>[3x]MPKIYTKTGDKGFSSTFTGERRPKDDQVFEAVGTTDELSSAIGFALELVTEKGHTFAEELQKIQCTLQDVGSALATPCSSAREAHLKYTTFKAGPI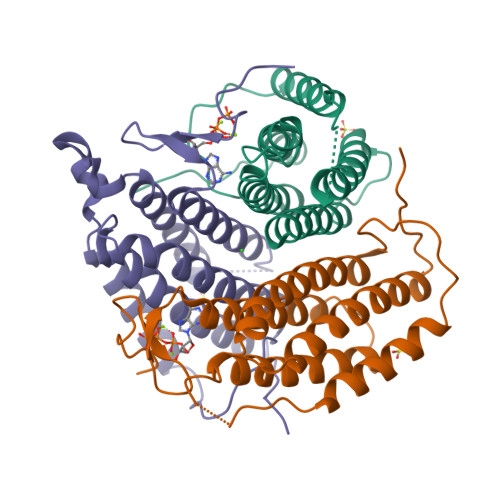LELEQWIDKYTSQLPPLTAFILPSGGKISSALHFCRAVCRRAERRVVPLVQMGETDANVAKFLNRLSDYLFTLARYAAMKEGNQEKIYMKNDPSAESEGL>[2x]ALSDRLELVSASEIRKLFDIAAGMKDVISLGIGEPDFDTPQHIKEYAKEALDKGLTHYGPNIGLLELREAIAEKLKKQNGIEADPKTEIMVLLGANQAFLMGLSAFLKDGEEVLIPTPAFVSYAPAVILAGGKPVEVPTYEEDEFRLNVDELKKYVTDKTRALIINSPCNPTGAVLTKKDLEEIADFV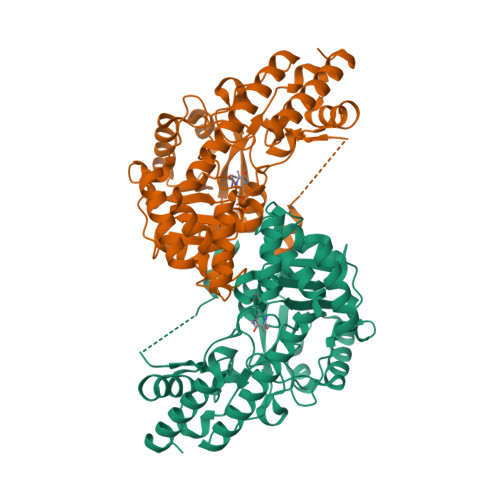VEHDLIVISDEVYEHFIYDDARHYSIASLDGMFERTITVNGFSKTFAMTGWRLGFVAAPSWIIERMVKFQMYNATCPVTFIQYAAAKALKDERSWKAVEEMRKEYDRRRKLVWKRLNEMGLPTVKPKGAFYIFPRIRDTGLTSKKFSELMLKEARVAVVPGSAFGKAGEGYVRISYATAYEKLEEAMERMERVLKERKLV>[11x]MSTSKRKRGDDSNWSKRVTKKKPSSAGLKRAGS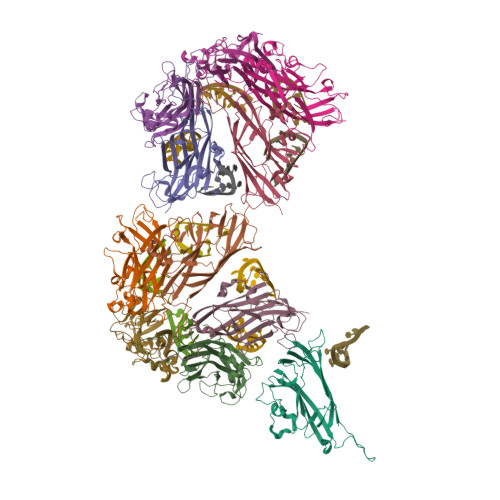KADRPSLQIQTLQHAGTTMITVPSGGVCDLINTYARGSDEGNRHTSETLTYKIAIDYHFVADAAACRYSNTGTGVMWLVYDTTPGGQAPTPQTIFAYPDTLKAWPATWKVSRELCHRFVVKRRWLFNMETDGRIGSDIPPSNASWKPCKRNIYFHKFTSGLGVRTQWKNVTDGGVGAIQRGALYMVIAPGNGLTFTAHGQTRLYFKSVGN>[2x]MSSNCTSTTAVAVAPLSASKTKTKKKHFVCQKVKLFRASEPILSVLMWGVNHTINELSNVPVPVMLMPDDFKAYSKIKVDNHLFNKENLPSRFKFKEYCPMVFRNLRERFGIDDQDYQN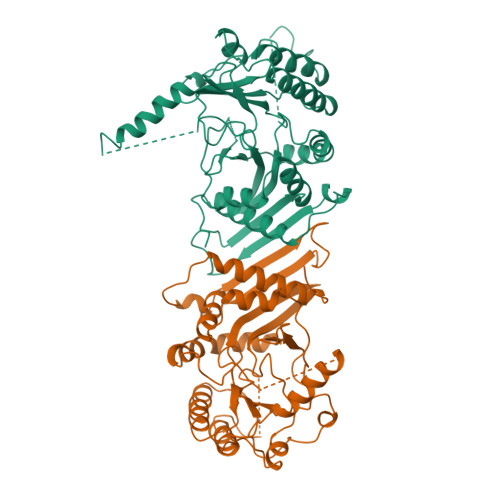SVTRSAPINSDSQGRCGTRFLTTYDRRFVIKTVSSEDVAEMHNILKKYHQFIVECHGNTLLPQFLGMYRLTVDGVETYMVVTRNVFSHRLTVHRKYDLKGSTVAREASDKEKAKDLPTFKDNDFLNEGQKLHVGEESKKNFLEKLKRDVEFLAQLKIMDYSLLVGIHDVDRAEQEEMEVEERAEDEECENDGVGGNLLCSYGTPPDSPGNLLSFPRFFGPGEFDPSVDVYAMKSHESSPKKEVYFMAIIDILTPYDTKKKAAHAAKTVKHGAGAEISTVNPEQYSKRFNEFMSNILT> EFMNAPLRGQVYRCDLGYG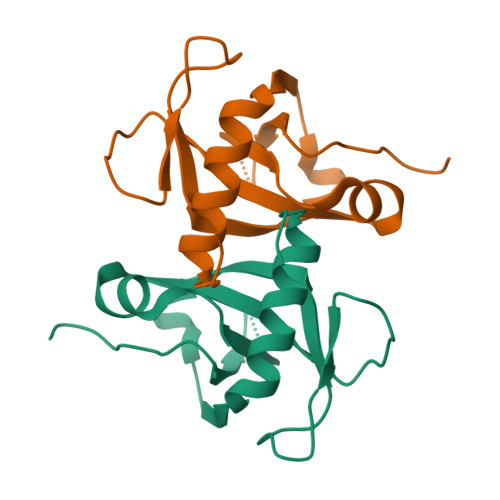AKPWLIVSNNARNRHTADVVAVRLTTTRRTIPTWVAMGPSDPLTGYVNADNIETLGKDELGDYLGEVTPATMNKINTALATALGLPWP> MENKIEVNNKDEMNKWFEEFKKGNGLVDTFTNSYSFCESVPNLDRFVFQMASATDDAQKDSIYASALVEATKFCAPIYECAWVSSTGIVKKGLEWFEKNAGTIKSWDESYTELKVEVPKIEQLADYQQAALKWRKDIGFRVNANTTALSHKVLAEYKVPGEIVMSVKEMLSDMIRRRNLILNRGGDENPRGPVSREHVEWCREFVKGKYIMAFNPPWGDINKSGRSGIALVATGLAKLAETEGKGVFDEAKKTVEALNGYLNKHKDEVDKASADSMITNLLKHIAKAQELYKNSSALRAQGAQIDTAFSSYYWLYKAGVTPETFPTVSQFLFELGKQPRGTKKMKKALLSTPLKWGKKLYELFADDSFQQNRIYMHPAVLTAGRISEMGVCFGTIPVANPDDAAQGSGHTKSILNLRTNTETNNPCAKTIVKLFEIQKTGFNIQDMDIVASEHLLHQ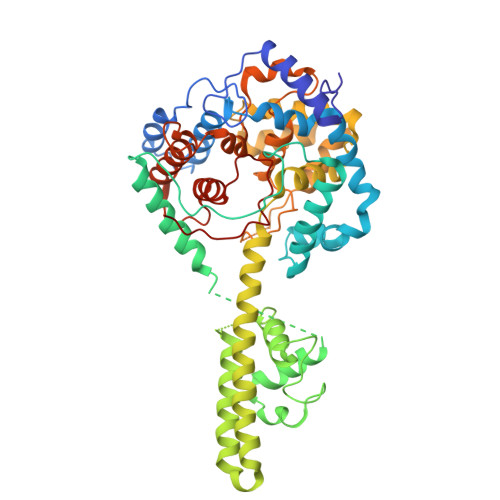SLVGKQSPFQNAYNVKGNATSANII>[2x]MLKQVEIFTDGSCLG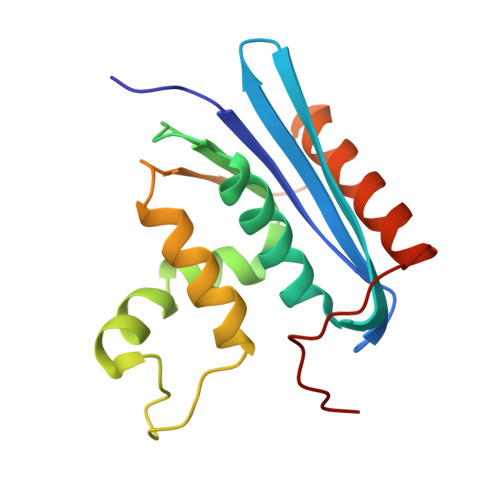NPGPGGYGAILRYRGREKTFSAGYTRTTNNRMALMAAIVALEALKEHCEVILSTDSQYVRQGITQWIHNWKARGWKTADKKPVKNVDLWQRLDAALGQHQIKWEWVKGHAGHPENERCDELARAAAMNPTLEDTGYQVEV> ANSTAELEELLMQRSLTDPQLQAAAAAAADFRILPDATVIKIGGQSVIDRGRAAVYPLVDEIVAARKNHKLLIGTGAGTRARHLY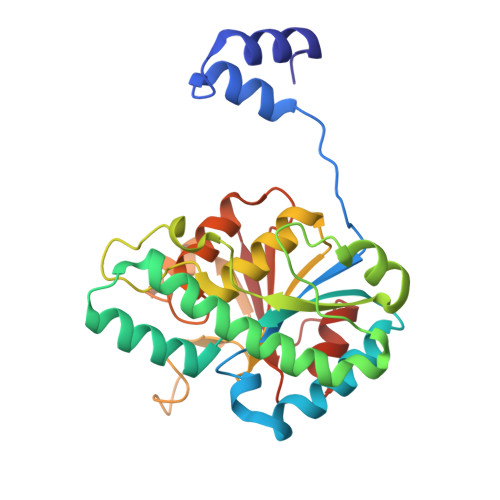SIAAGLGLPAGVLAQLGSSVADQNAAMLGQLLAKHGIPVVGGAGLSAVPLSLAEVNAVVFSGMPPYKLWMRPAAEGVIPPYRTDAGCFLLAEQFGCKQMIFVKDEDGLYTANPKTSKDATFIPRISVDEMKAKGLHDSILEFPVLDLLQSAQHVREVQVVNGLVPGNLTRALAGEHVGTIITAS> FRAIIESPEGAGHVGYQYRRNTGSTMRMVSDVLDERVSLWDFHCDPSGNVIQPGPNVDSRQYLQAAIDYVSSNGGGTITIPAGY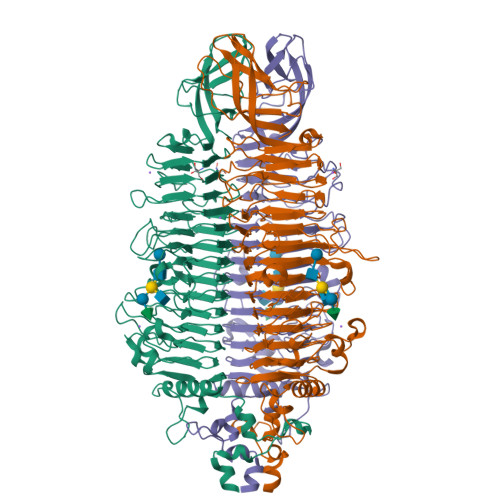TWYLGSYGVGGIAGHSGIIQLRSNVNLNIEGRIHLSPFFDLKPFQVFVGFDNGDPASSGNLENCHIYGHGVVDFGGYEFGASSQLRNGVAFGRSYNCSVTGITFQNGDVTWAITLGWNGYGSNCYVRKCRFINLVNSSVNADHSTVYVNCPYSGVESCYFSMSSSFARNIACSVALHQHDTFYRGSTVNGYCRGAYVVMHAAEAAGAGSYAYNMQVENNIAVIYGQFVILGSDVTATVSGHLNDVIVSGNIVSIGERAAFSAPFGAFIDIGPDNSGASNVQDIQRVLVTGNSFYAPANITDSAAITLRANLNGCTFIANNFDCRYMVYNAPGTTSPVVQNLVWDKSNVIGGTHANQRAGQNLFDMQFASVVNSTIEVQLSCEDLSMFSCILFPASCQLSYSKITVDSAWTKSMSNTAVFEGNQQAGANVYVSYPATVNLTSYNTQGAVPFFSTDTNYAWVTSAYSLSINENLDFSPPATYTNKANGQLVGVGYNEIGGVRSVSVRLMLQRQV> MEPAPSEVRLAVREAIHALSSSEDGGHIFCTLESLKRYLGEMEPPALPREXXXXXXXXXXK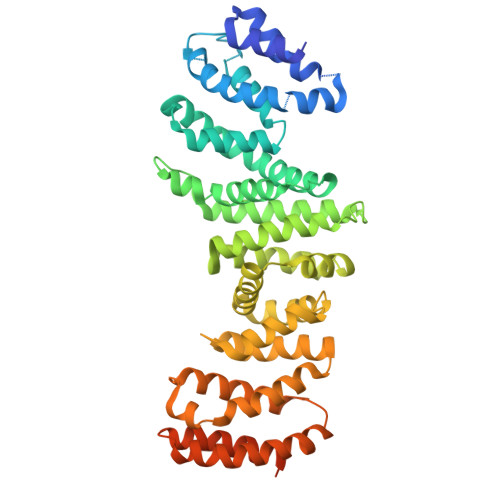EEFASAHFSPVLRCLASRLSPAWLELLPHGRLEXXXXXXXXELWASFFLEGPADQAFLVLMETIEGAAGPSFRLMKMARLLARFLREGRLAVLMEAQCRQQTQPGFILLRETLLGKVVXXXXXXXXXXXXXXXXXXALPDHLGNRLQQENLAEFFPQNYFRLLGEEVVRVLQAVVDSLQGGLDSSVSFVSQVLGKACVHGRQQEILGVLVPRLAALTQGSYLHQRVCWRLVEQVPDRAMEAVLTGLVEAALGPEVLSRLLGNLVVKNKKAQFVMTQKLLFLQSRLTTPMLQSLLGHLAMDSQRRPLLLQVLKELLETWGSSSAIRHTPLPQQRHVSKAVLICLAQLGEPELRDSRDELLASMMAGVKCRLDSSLPPVRRLGMIVAEVVSARIHPEGPPLKFQYEEDELSLELLALASPQPAGDGASEAGT> MGSLVCVGTGLQLAGQISVLSRSYIEHADIVFSLLPDGFSQRWLTKLNPNVINLQQFYAQNGEVKNRRDTYEQMVNAILDAVRAGKKTVCALYGHPGVFACVSHMAITRAKAEGFSAKMEPGISAEACLWADLGIDPGNSGHQSFEASQFMFFN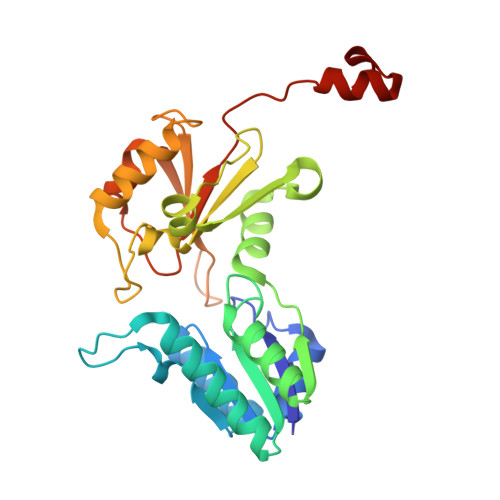HVPDPTTHLLLWQIAIAGEHTLTQFHTSSDRLQILVEQLNQWYPLDHEVVIYEAANLPIQAPRIERLPLANLPQAHLMPISTLLIPPAKKLEYNYAILAKLGIGPEDLG> MKVNNTIVVSIGQAGNQIAASFWKTVCLEHGIDPLTGQTAPGVAPRGNWSSFFSKLGESSSGSYVPRAIMVDLEPSVIDNVKATSGSLFNPANLISRTEGAGGNFAVGYLGAGREVLPEVMSRLDYEIDKCDNVGGIIVLHAIGGGTGSGFGALLIESLKEKYGEIPVLSCAVLPSPQVSSVVTEPYNTVFA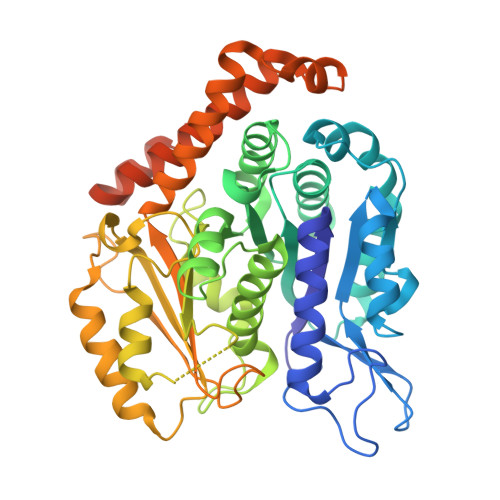LNTLRRSADACLIFDNEALFDLAHRKWNIESPTVDDLNLLITEALAGITASMRFSGFLTVEISLRELLTNLVPQPSLHFLMCAFAPLTPPDRSKFEELGIEEMIKSLFDNGSVFAACSPMEGRFLSTAVLYRGIMEDKPLADAALAAMREKLPLTYWIPTAFKIGYVEQPGISHRKSMVLLANNTEIARVLDRICHNFDKLWQRKAFANWYLNEGMSEEQINVLRASAQELVQSYQVAEESGAKAKVQDSAGDTGMRAAAAGVSDDARGSMSLRDLVDRRR>[14x]GSMNLIPTVIETTNRGERAYDIYSRLLKDRIIMLGSQIDDNVANSIVSQLLFLQAQDSEKDIYLYINSPGGSVTAGFAIYDTIQHIKPDVQTICIGMAASMGSFLLAAGAK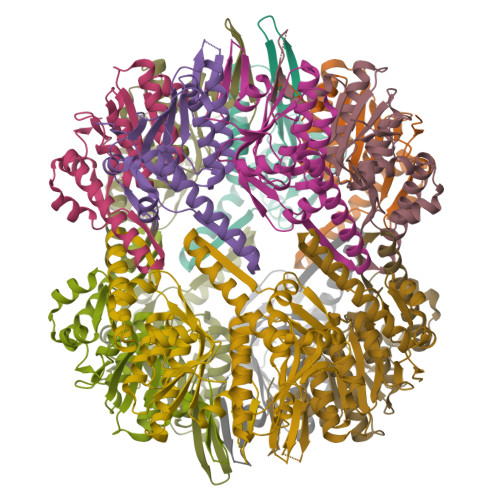GKRFALPNAEVMIHQPLGGAQGQATEIEIAANHILKTREKLNRILSERTGQSIEKIQKDTDRDNFLTAEEAKEYGLIDEVMVPETK> RTVVRTFDFELSGYPDET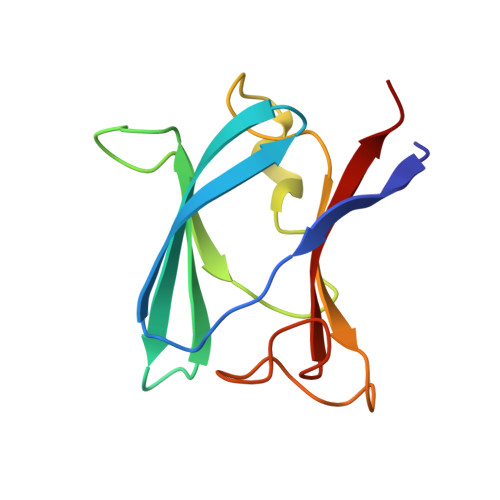FRVVLDSVTYELRFMWNERDESWFMSLGDIGAQRPTITSKLTCYSDILAPYRYLDNVPDGNLYLWPLGDIRTRAGRFNIGPLKGIQMTYSSLIE6,8-bis(fluoranyl)chromene | 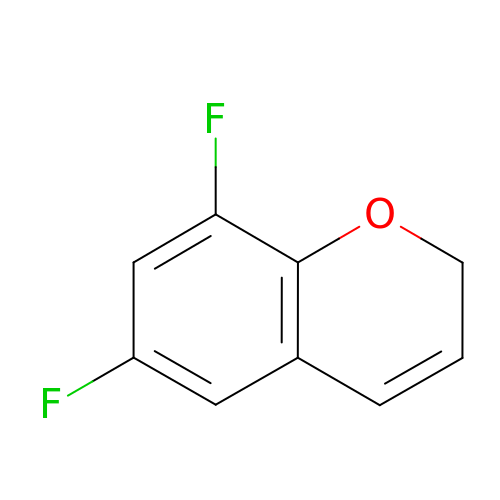C9 H6 F2 O | DRQKJKGKLYCHHB-UHFFFAOYSA-N VanR belongs to the PadR family of regulatory proteins and has been proved to specifically respond to its effetor vanillic acid, a hydroxytyrosol analog. In C. glutamicum, VanR regulates the expression of the vanABK operon, which is responsible for the catabolism of vanillic acid. In the absence of vanillic acid, the VanR protein binds to a 28-bp operator sequence downstream of +1 position of the PvanABK promoter and represses the transcription of the vanABK operon. When vanillic acid is present, it binds to the VanR protein, inducing a conformational change which releases the promoter DNA, thus activating the operon transcription.

To facilitate VanR engineering, we determined the crystal structure of VanR complexed with vanillic acid. VanR functions as a homodimer and each monomer consists of an N-terminal winged helix-turn-helix (wHTH) domain which interacts with operator DNA, and a C-terminal homodimerization domain. Electronic densities of vanillic acids were found in the interface of two subunits. Vanillic acid binds to a hydrophobic interdomain pocket formed by V29, Y168, M133, L145, and H142 from subunit A and Y103 of subunit B. Besides hydrophobic interaction, polar contacts largely contribute to the recognition of vanillic acid by VanR. Specifically, the carboxyl group of vanillic acid is electrostatically stabilized by salt bridges with R148 of subunit A and by hydrogen bond with the side chain of Y103 of subunit B. Furthermore, the hydroxyl and methoxyl groups on the benzene ring of vanillic acid form two hydrogen bonds with the side chains from Y168 of subunit A. Those three residues were highly conserved in different bacteria, suggesting they are essential for ligand recognition. To alter the effector specificity of VanR, amino acid residues Y103, R148, and Y168, were chosen for simultaneous site-saturation mutagenesis. The sequencing results revealed amino acid substitutions (Y103L, R148L and Y168M) in HyT12. The crystal structure of the regulatory protein VanR from C. glutamicum complexed with its inducer was elucidated based on which a hydroxytyrosol biosensor was developed by altering the induction specificity of VanR.

>[2x]MTLRSALLALLSSGPLTGYDASQRFGASVGFVWSGSDSQIYPELRKMEAEELLVGSDVPWGSKGATKTEYALSEKGWEALRKAWYEPVTYGPTRDPARLKAAYFEVGTNGDARRHLRAHIAHFEQQKIQSESMIDELKAKTHPTLARRLERSPKKEHERIVAFKVLAYEGQIARAQAEIEWAEKGLKLLDTL> SMDLRVQELIKLICNVQAMEEMMMEMKYNTKKAPLGKLTVAQIKAGYQSLKKIEDCIRAGQHGRALMEACNEFYTRIPHDFGLRTPPLIRTQKELSEKIQLLEALGDIEIAIKLVKTELQSPEHPLDQHYRNLHCALRPLDHESYEFKVISQYLQSTHAPTHSDYTMTLLDLFEVEKDGEKEAFREDLHNRMLLWHGSRMSNWVGILSHGLRIAHPEAPITGYMFGKGIYFADMSSKSANYCFASRL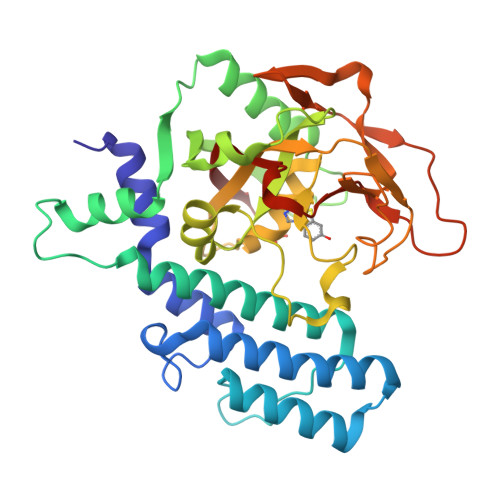KNTGLLLLSEVALGQCNELLEANPKAEGLLQGKHSTKGLGKMAPSSAHFVTLNGSTVPLGPASDTGILNPDGYTLNYNEYIVYNPNQVRMRYLLKVQFNFLQLW>MRAKIPSEEVAVKLNEWYKLIRAFEADQAEALKQEIEYDLEDMEENQDLLLYFSLMEFRHRIMLDKLMPVKDSDTKPPFSDMLNEIESNQQKLTGLLEYYFYYFRGMYEFKQKNFILAIDHYKHAEEKLEYVEDEIEKAEFLFKVAEVYYHIKQTYFSMNYASQALDIYTKYELYGRRRVQCEFIIAGNLTDVYHHEKALTHLCSALEHARQLEEAYMIAAAYYNVGHCKYSLGDYKEAEGYFKTAAAIFEEHNFQQAVQAVFSLTHIYCKEG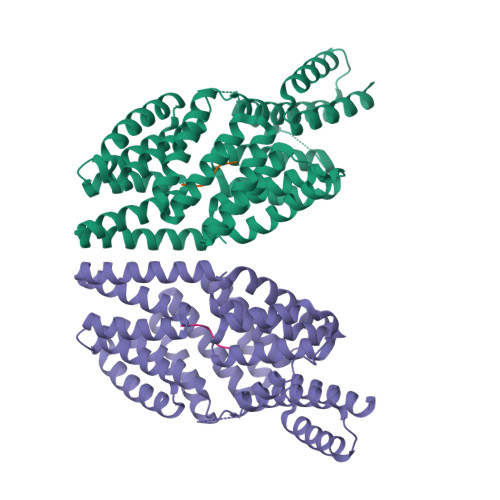KYDKAVEAYDRGIKSAAEWEDDMYLTKFRLIHELYLGSGDLNVLTECFDLLESRQLLADAEDLLHDTAERFNQLEHYESAAFFYRRLMNIKKKLAEQRFQ[2x];>[2x]ERGMT>GDEPSDLEELEKFAKTFKQRRIKLGFTQGDVGLAMGKLYGNDFSQTTISRFEALNLSFKNMCKLKPLLEKWLNDAESSPSDPSVSTPSSYPSLSEVFGRKRKKRTSIETNIRLTLEKRFQDNPKPSSEEISMIAEQLSMEKEVVRVWFCNRRQKEKRINC[2x];>GMSEKPKVYQGVRV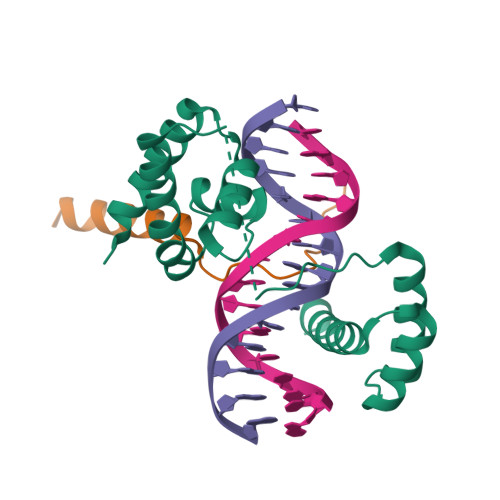KITVKELLQQRRAHQAASGGTRSGG[2x]> QLEAS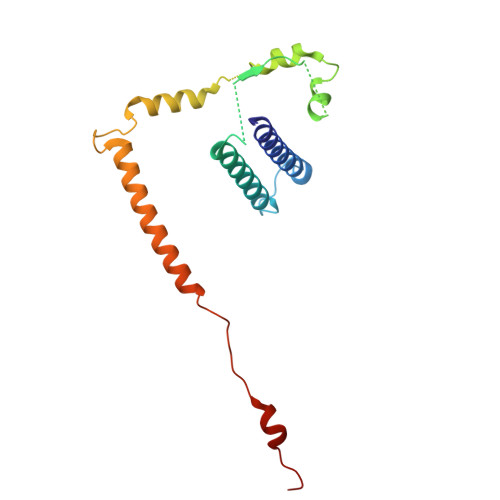LDALLNQVADLKNSLGSFIYKLENEYDRLTWPSVLDSFALLSGQLNTLNKVLKHEKTPLFRNQVIIPLVLSPDRDEDLMRQTEGRVPVFSHEVVPDHLRTKPDPEVEEQEKQLTTDAARIGADAAQKQIQSLNKMCSNLLEKISKEERESESGGLRPNKQTFNPGDTNALVAAVA>[2x]PIKVYGQVSLNDSHNQMVVHWAGEKSNVIVALARDSLALARPKSSDVYVSYDYGKSFKKISDKLNFGLGNRSEAVIAQFYHSPADNKRYIFADAYAQYLWITFDFCNTLQGFSIPFRAADLLLHSKASNLLLGFDRSHPNKQLWKSDDFGQTWIMIQEHVKSFSWGIDPYDKPNTIYIERHEPSGYSTVFRSTDFFQSRENQEVILEEVRDFQLRDKYMFATKVVHLLGSEQQSSVQLWVSFGRKPMRAAQFVTRHPINEYYIADASEDQVFVCVSHSNNRTNLYISEAEGLKFSLSLENVLYY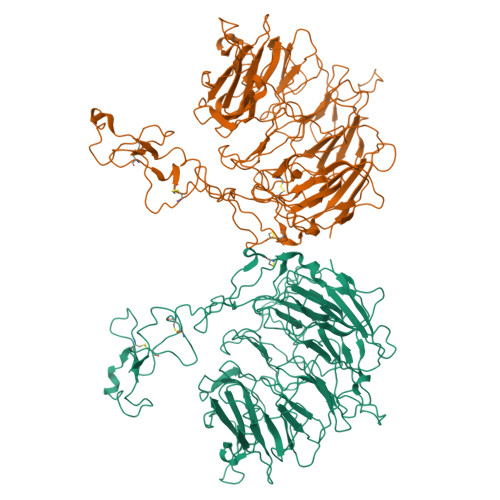SPGGAGSDTLVRYFANEPFADFHRVEGLQGVYIATLINGSMNEENMRSVITFDKGGTWEFLQAPAFTGYGEKINCELSQGCSLHLAQRLSQLLNLQLRRMPILSKESAPGLIIATGSVGKNLASKTNVYISSSAGARWREALPGPHYYTWGDHGGIITAIAQGMETNELKYSTNEGETWKTFIFSEKPVFVYGLLTEPGEKSTVFTIFGSNKENVHSWLILQVNATDALGVPCTENDYKLWSPSDERGNECLLGHKTVFKRRTPHATCFNGEDFDRPVVVSNCSCTREDYECDFGFKMSEDLSLEVCVPDPEFSGKSYSPPVPCPVGSTYRRTRGYRKISGDTCSGGDVEARLEGELVPC>GSTGSPPGPPGVVIVEEITESTATLSWSPATDNHSPISSYNLQARSPFSLGWQTVKTVPEVITGDMESAMAVDLNPWVEYEFRVVATNPIGTGDPSIPSRMIRTNEAVPKTAPSNVSGRSGRRHELVIAWEPVSEEFQNGEGFGYIVAFRPNGTRGWKEKMVTSSEASKFIYRDESVPPLTPFEVKVGVYNNKGDGPFSQIVVICSAEGEPTAAPTDVTATSVSVSEIFVVWKHVKESLGRPQGFEISYWKDTEPED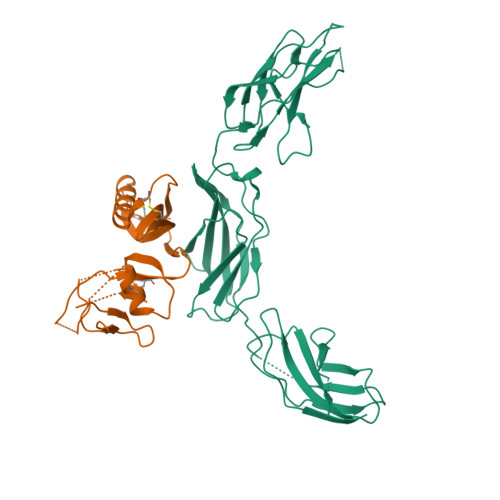SVETVRTRGNESFVMLTGLEGNTLYHLTVRAYNGAGYGPPSREASTTTKR[2x];>GPGSEVPTDGNAGLLAEPQIAMFCGKLNMHMNVQNGKWESDPSGTKTCIGTKEGILQYCQEVYPELQITNVVEANQPVTIQNWCKRGRKQCKTHTHIVIPYRCLVGEFVSDALLVPDKCKFLHQERMDVCETHLHWHTVAKETCSEKSTNLHDYGMLLPCGIDKFRGVEFVCCPLA[2x]> GANETTKQESPVVDTDINAVTNYIVGMC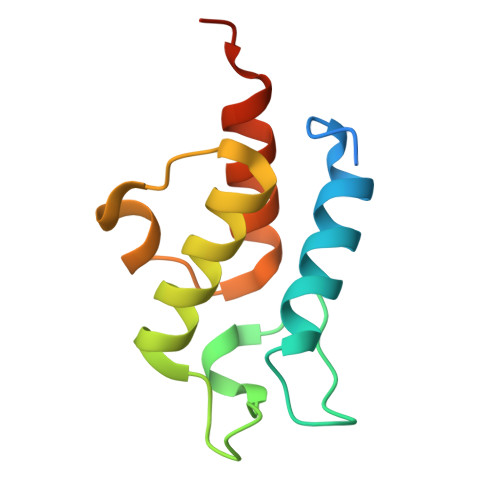QKFLQKGEKVTPSSKLEELRTREDRLWDCLDTVEFVLDVEEIFDVTVPDEVADNFQTLQEIADFVVSERAKAGKFMKDQ>MTDIINKLQAFADANPQSIAVRHTTDELTYQQLMDESSKLAHRLQGSKKPMILFGHMSPYMIVGMIGAIKAGCGYVPVDTSIPEDRIKMIINKVQPEFVFNTTDESFESLEGEVFTIEDIKTSQDPVIFDSQIKDNDTVYTIFTSGSTGEPKGVQIEYASLVQFTEWMLELNKSGNKQQWLNQAPFSFDLSVMAIYPCLASGGTLNLVDKNMINKPKLLNEMLTATPINIWVSTPSFMEMCLLLPTLNEEQYGSLNEFFFCGEILPHRAAKALVSRFPSATIYNTYGPTEATVAVTSIQITQEILDQYPTLPVGVERLGARLSTTDDGELVIEGQSVSLGYLKNDQKTAEVFNFDDGIRTYHTGDKAKFENGQWFIQGRIDFQIKLNGYRMELEEIETQLRQSEFVKEAIVVPVYKNDKVIHLIGAIVPTTEVTDNAEMTKNIKNDLKSRLPEYMIPRKFEWMEQLPLTSNGKIDRKKIAEVING[4x]

d-Alanylation of the teichoic acids of the Gram-positive bacterial cell wall plays crucial roles in bacterial physiology and virulence. Hence, the d-alanylation pathway has emerged as a promising antibacterial target against drug-resistant S. aureus. d-Alanylation of teichoic acids is mediated via the action of four proteins encoded by the dlt operon, DltABCD, all four of which are essential for the process. Similar to other adenylate-forming enzymes, DltA utilizes several distinct structural conformations to catalyze two sequential reactions: (i) adenylation of d-Ala at the expense of ATP followed by (ii) thioesterification of the 4′-phosphopantetheinyl (Ppant) prosthetic group of the d-Ala carrier protein DltC. Here, the crystal structure of DltA from the methicillin-resistant S. aureus strain Mu50 is presented, which reveals the unique molecular details of the catalytic center and the role of the P-loop.

DltA from S. aureus (SaDltA) was crystallized in the presence of ATP and Mg2+. The monoclinic crystal, belonging to space group P21, contains four DltA molecules (chains A, B, C and D) in the asymmetric unit. Subsequent d-Ala adenylate formation and breakage of the ATP phosphodiester bond result in a 140° rotation of the C-terminal subdomain towards the ‘thiolation conformation’, in which the Ppant group of DltC can approach the active site of DltA for loading of d-Ala to complete the reaction. The SaDltA structure features the canonical adenylation conformation, allowing it to grasp the ATP substrate and Mg2+ ion in the active site that lies between the N- and C-terminal lobes and posing it for the d-alanine adenylation reaction with the Ppant substrate channel blocked by the loop (Ppant blocking loop; residues 463–476) in the C-terminal lobe. Clear electron density for ATP and magnesium in the active-site pocket is observed in all chains in the asymmetric unit. The P-loop of DltA has an amino-acid composition similar to that of the P-loop or Walker A motif found in other adenylate-forming enzymes; thus, the loop has been suggested to bind ATP or pyrophosphate, despite the lack of direct structural data to support this assumption. In chains A and B of SaDltA we observed clear electron density allowing us to unambiguously assign the residues of the P-loop, whereas the electron density of the corresponding residues in chains C and D was very weak and we could not model four residues (residues 148–151), indicating significant flexibility of the region.> HMASKPVWGDVNCDGDVNVADVVLLNKWLNNNADYAMT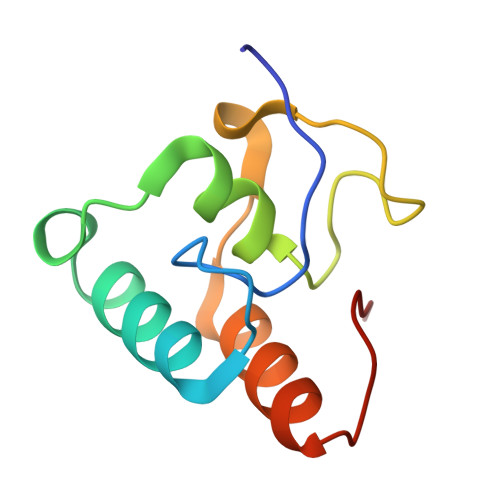DQGKVNADCFNPQDANGGAVDASKVDLTKTDSDAIIKSVVHLITLPAKG> GEFFAVSNMLEALDSGKFGSVSKELEEIADMRMDLVKRSIWLYPSLAY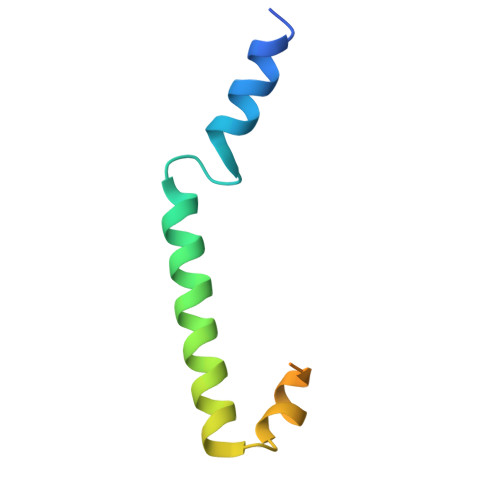TVFEAEKTMDGGGGSDYKDDDDK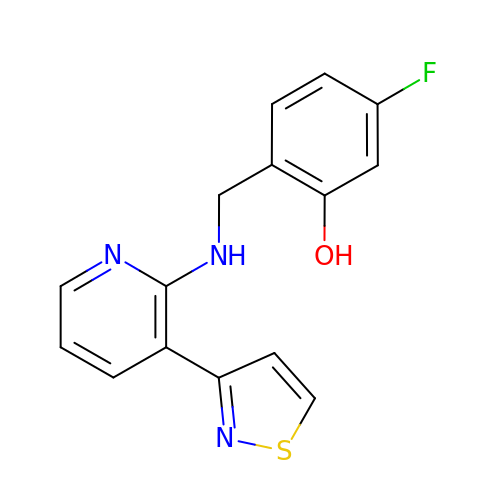5-fluoro-2-({[(3M)-3-(1,2-thiazol-3-yl)pyridin-2-yl]amino}methyl)phenol | C15 H12 F N3 O S | VHMHZWAZTGHNTQ-UHFFFAOYSA-N> MTDFLKIELIGRDGSHWVLSGPGMGQQGVTLNPNLQQFYDAPVKTLYVPGPFGEEYAGKRVQRREIVFSVQAYDEDPDTWSTVDSLWRWAWDYDEESELRVSTSDGTRFLKVRLMEEPKPYYEKDPHITADNPIVMTVTATFPYWQDEP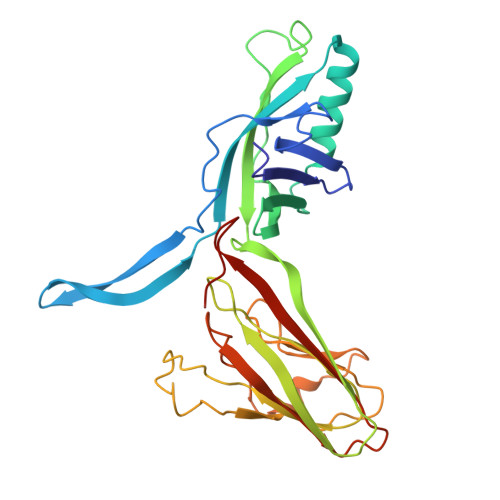EELIWTTLSTEDMTRFPVRNDGDVPVWLKWTLTAPGLWILPDFSWGNDMYSRGREDLGRTVAMPELVAGEHVSVDSDPRVQTLIAVNGMPTQNRWKGNDLLYPLMPGKGAEIPVQLKNAPEGGACKLTRPRWYSRPWSRPGVRLNG> ITYEAREEAAQQSVNRV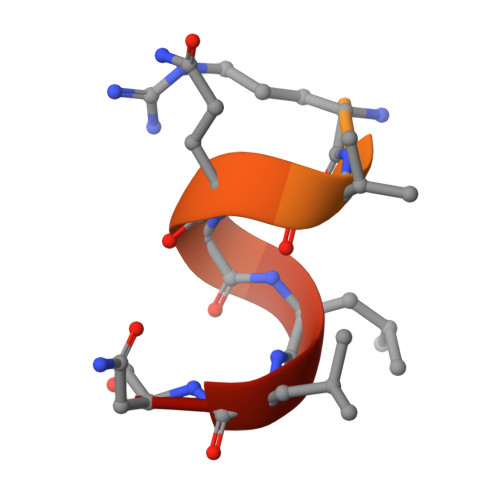QALLNG>MHHHHHHRKRPEVILKLALSADGMIGRKGAGQVAITGPVSRAQSHILRAQADIILIGIETALADDPVLNCRLPGLEQRSPVRVVLDGGLRLPLSSRLVRSADTQPLWVACGEEAPDERRAALGAAGCRILATETHDGRIALPELLDDLAAQGIASVLVEGGAGVAKSFLDEKLVDRLIIFRSPLVIGAADGVAVEGLETHIASEFKILRRMRYADDACA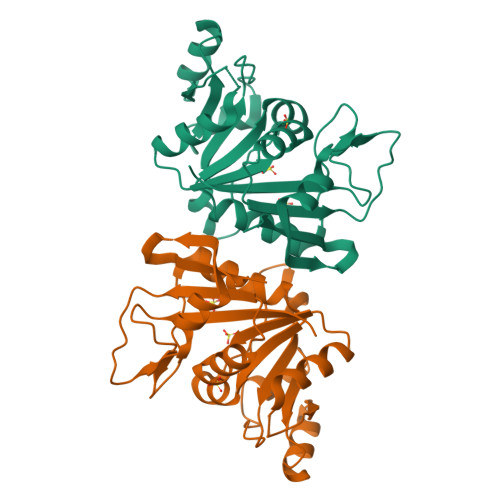EYVRNT[4x]> MTVLKMTDLDLQGKRVLIREDLNVPVKDGVVTSDARILASLPTIKLALEKGAAVMVCSHLGRPTEGEFSAENSLKPVADYLSKALGREVPLVSDYLNGVDVKAGDIVLFENVRFNKGEKKNADELAKQYAALCDVFVMDAFGTAHRAEGSTHGVAKFAKVAAAGPLLAAELDALGKALGAPAKPMAAIVAGSKVSTKLDVLNSLSQICDLLIVGGGIADTFLAAAGHPVGKSLYEPDLLDTARAIAAKVNVPLPTDVVVAKEFAESAEATVKLIADVAADDMILDIGPQTAEHF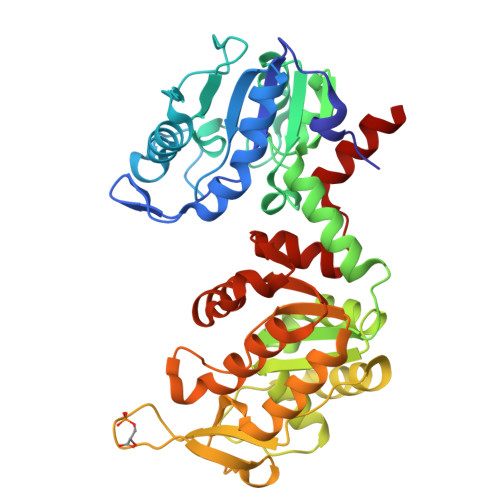AQLLKTSKTILWNGPVGVFEFDQFGNGTKVLAKAIADSAAFSIAGGGDTLAAIDKYGVADQISQISTGGGAFLEFVEGKVLPAVEVLESRAKA> MSILTRWLLIPPVNARLIGRYRDYRRHGASAFSATLGCFWMILAWIFIPLEHPRWQRIRAEHKNLYPHINASRPRPLDPVRYLIQTCWLLIGASRKETPKPRRRAFSGLQNIRGRYHQWMNELPERVSHKTQHLDEKKELGHLSAGARRLILGIIVTFSLILALICVTQPFNPLAQFIFLMLLWGVALIVRRMPGRFSALMLIVLSLTVSCRYIWWRYTSTLNWDDPVSLVCGLILLFAETYAWIVLVLGYFQVVWPLNRQPVPLPKDMSLWPSVDIFVPTYNEDLNVVKNTIYASLGIDWPKDKLNIWILDDGGREEFRQFAQNVGVKYIARTTHEHAKAGNINNALKYAKGEFVSIFDCDHVPTRSFLQMTMGWFLKEKQLAMMQTPHHFFSPDPFERNLGRFRKTPNEGTLFYGLVQDGNDMWDATFFCGSCAVIRRKPLDEIGGIAVETVTEDAHTSLRLHRRGYTSAYMRIPQAAGLATESLSAHIGQRIRWARGMVQIFRLDNPLTGKGLKFAQRLCYVNAMFHFLSGIPRLIFLTAPLAFLLLHAYIIYAPALMIALFVLPHMIHASLTNSKIQGKYRHSFWSEIYETVLAWYIAPPTLVALINPHKGKFNVTAKGGLVEEEYVDWVISRPYIFLVLLNLVGVAVGIWRYFYGPPTEMLTVVVSMVWVFYNLIVLGGAVAVSVESKQVRRSHRVEMTMPAAIAREDGHLFSCTVQDFSDGGLGIKINGQAQILEGQKVNLLLKRGQQEYVFPTQVARVMGNEVGLKLMPLTTQQHIDFVQCTFARADTWALWQDSYPEDKPLESLLDILKLGFRGYRHLAEFAPSSVKGIFRVLTSLVSWVVSFIPRRPERSETAQPSDQALAQQGSARSSGRTGLEFEEFYPYDVPDYAADYKDDDDKRS;>MTQFTQNTAMPSSLWQYWRGLSGWNFYFLVKFGLLWAGYLNFHPLLNLVFAAFLLMPLPRYSLHRLRHWIALPIGFALFWHDTWLPGPESIMSQGSQVAGFSTDYLIDLVTRFINWQMIGAIFVLLVAWLFLSQWIRITVFVVAILLWLNVLTLAGPSFSLWPAGQPTTTVTTTGGNAAATVAATGGAPVVGDMPAQTAPPTTANLNAWLNNFYNAEAKRKSTFPSSLPADAQPFELLVINICSLSWSDIEAAGLMSHPLWSHFDIEFKNFNSATSYSGPAAIRLLRASCGQTSHTNLYQPANNDCYLFDNLSKLGFTQHLMMGHNGQFGGFLKEVRENGGMQSELMDQTNLPVILLGFD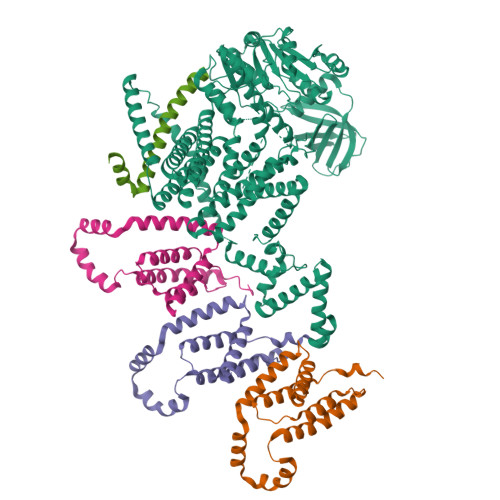GSPVYDDTAVLNRWLDVTEKDKNSRSATFYNTLPLHDGNHYPGVSKTADYKARAQKFFDELDAFFTELEKSGRKVMVVVVPEHGGALKGDRMQVSGLRDIPSPSITDVPVGVKFFGMKAPHQGAPIVIEQPSSFLAISDLVVRVLDGKIFTEDNVDWKKLTSGLHKQHRSPRTQMQ[3x];> TPATQPLINAEPAVAAQTEQNPQVGQVMPGVQGADAPVVAQNGPSRDVKLTFAQIAPPPGSMVLRGINPNGSIEFGMRSDEVVTKAMLNLEYTPSPSLLPVQSQLKVYLNDELMGVLPVTKEQLGKKTLAQMPINPLFITDFNRVRLEFVGHYQDVCENPASTTLWLDVGRSSGLDLTYQTLNVKNDLSHFPVPFFDPRDNRTNTLPMVFAGAPDVGLQQASAIVASWFGSRSGWRGQNFPVLYNQLPDRNAIVFATNDKRPDFLRDHPAVKAPVIEMINHPQNPYVKLLVVFGRDDKDLLQAAKGIAQGNILFRGESVVVNEVKPLLPRKPYDAPNWVRTDRPVTFGELKTYEEQLQSSGLEPAAINVSLNLPPDLYLMRSTGIDMDINYRYTMPPVKDSSRMDISLNNQFLQSFNLSSKQEANRLLLRIPVLQGLLDGKTDVSIPALKLGATNQLRFDFEYMNPMPGGSVDNCITFQPVQNHVVIGDDSTIDFSKYYHFIPMPDLRAFANAGFPFSRMADLSQTITVMPKAPNEAQMETLLNTVGFIGAQTGFPAINLTVTDDGSTIQGKDADIMIIGGIPDKLKDDKQIDLLVQATESWVKTPMRQTPFPGIVPDESDRAAETRSTLTSSGAMAAVIGFQSPYNDQRSVIALLADSPRGYEMLNDAVNDSGKRATMFGSVAVIRESGINSLRVGDVYYVGHLPWFERLWYALANHPILLAVLAAISVILLAWVLWRLLRIISRRRLNPDNE~{N}-[4-[5-[3-[(dimethylamino)methyl]phenyl]-6-(1-methylpyrazol-4-yl)furo[2,3-d]pyrimidin-4-yl]oxyphenyl]-2-(4-fluorophenyl)-1-methyl-3-oxidanylidene-pyrazole-4-carboxamide | C36 H31 F N8 O4 | 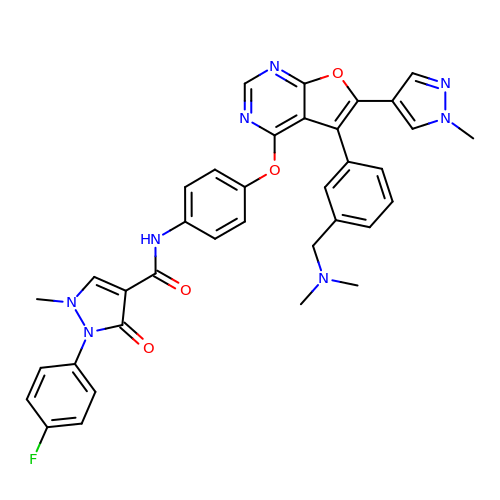WOAZQVRBSBTOAN-UHFFFAOYSA-N> ELLDPCGYISPESPVVQLHSNFTAVCVLKEKCMDYFHVNANYIVWKTNHFTIPKEQYTIINRTASSVTFTDIASLNIQLTCNILTFGQLEQNVYGITIISGLPPEKPKNLSCIVNEGKKMRCEWDGGRETHLETNFTLKSEWATHKFADCKAKRDTPTSCTVDYSTVYFVNIEVWVEAENALGKVTSDHINFDPVYKVKPNPPHNLS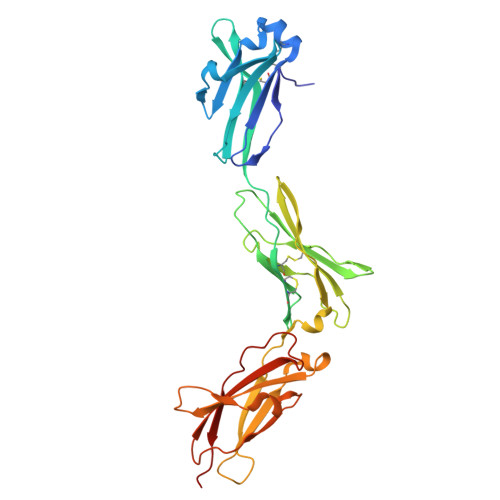VINSEELSSILKLTWTNPSIKSVIILKYNIQYRTKDASTWSQIPPEDTASTRSSFTVQDLKPFTEYVFRIRCMKEDGKGYWSDWSEEASGITYEDR>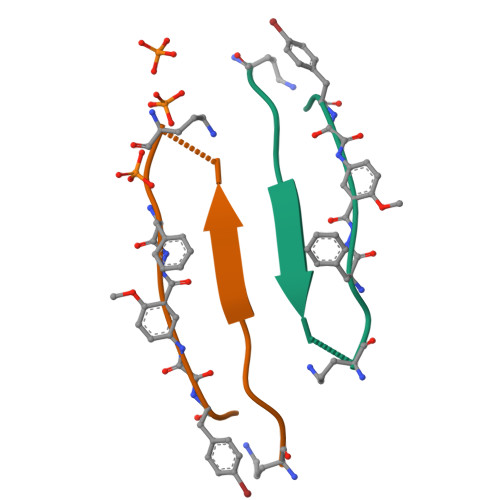[4x]ASVQIVYKAEFXYK>[2x]MKPHNSEKYFVKNGQPHFLISGEVHYFRINPKLWRNHLQLLKQTGADTVSTYIPWDWHEIEEDDFDFEGKTHPARNLIRFIKLCKEENLDLIVKPGPYILAEYENQGLPSWLLKKLSKNAFALDENGNVISPDLVSYLSDEFLEYTFKWYDKVMPIISKHQKEHYGPITMMQLCNEIGVFQWLSGKSDYNPKVINLYKEFIIQRYKTIEKLNSVYSTNYNSFDDLKAPSGKIKLRSDYCAYFDFHLFFREYYNKYISILKNKIRSFGINIKLTHNIPGWIYGNASELPMLISTYSEIMKNHPDIIFGLDHIPEFVSFRNAHSDLACNKILEAMQPEAPVWAAQFQAGTREHHVKAYAKDLETFYIASLAHGIKGFNYYMFSQ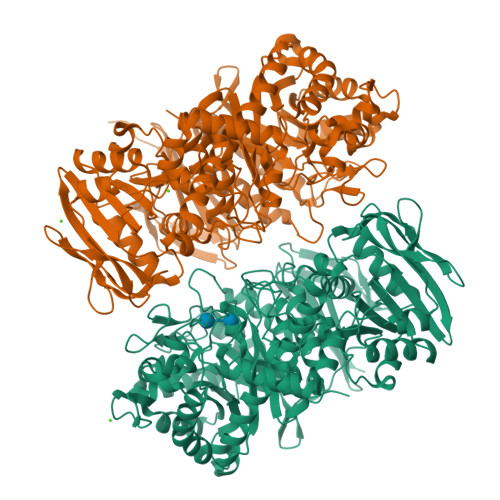GINPEGKGFYGKTFYFQTALDAASNKLALYDSIKKVNRFIRKEQKDLLRTNVNSEICVGFYKPYFFTELISSQLLKEKKLNVEELGLYIDPRFLREEILFNGLLRGLQTLNYNYDVVDLENCDLKSLTAYKQLWITSAEFMDAETQNLLSEFVLNGGNLILYPAVPTLDNYLNRCEILKNNFGIEFITKDSSHKVSAFGIEDVFTAFSKKQIYNDTNSKPIAFTQENEICGIRKKIGKGELTILGFAFGYTSDEHLELIDKLVKLNKIKRELFVSDKDIQFVVRENNKSRYIFFLNYHNERKTFNYRKSSELKKKKSEEISIAPFSYKVIKENKLEHHHHHH> PRRRDPQDDVYLDITDRLCFAILYSRPKSASNVHYFSIDNELEYENFYADFGPLNLAMVYRYC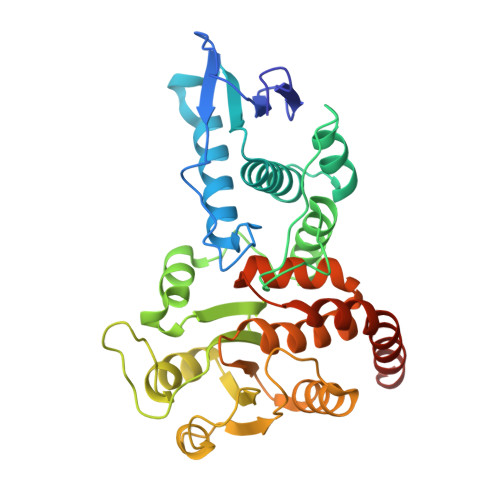CKINKKLKSITMLRKKIVHFTGSDQRKQANAAFLVGCYMVIYLGRTPEEAYRILIFGETSYIPFRDAAYGSCNFYITLLDCFHAVKKAMQYGFLNFNSFNLDEYEHYEKAENGDLNWIIPDRFIAFCGPHSRARLESGYHQHSPETYIQYFKNHNVTTIIRLNKRMYDAKRFTDAGFDHHDLFFADGSTPTDAIVKEFLDICENAEGAIAVHCKAGLGRTGTLIACYIMKHYRMTAAETIAWVRICRPGSVIGPQQQFLVMKQTNLWLEGDYFRQKLKGQENGQH[(1~{R},5~{S},6~{R},8~{R},9'~{S})-9'-(aminomethyl)-8-(6-aminopurin-9-yl)-2'-bromanyl-5'-[3-oxidanylidene-3-(1,3-thiazol-2-ylamino)propoxy]spiro[2,4,7-trioxa-3-boranuidabicyclo[3.3.0]octane-3,7'-8-oxa-7-boranuidabicyclo[4.3.0]nona-1(6),2,4-triene]-6-yl]methyl 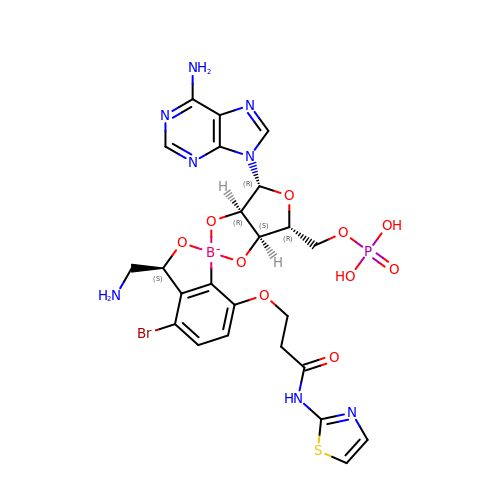dihydrogen phosphate | C24 H26 B Br N8 O10 P S | WVJYJHILOSTTGL-NCOZZQORSA-N> AFVVTDNCIKCKYTDCVEVCPVDCIYEGPNFLVIHPDECIDCALCEPECPAQAIFSEDEVPEDMQEFIQLNAELAEVWPN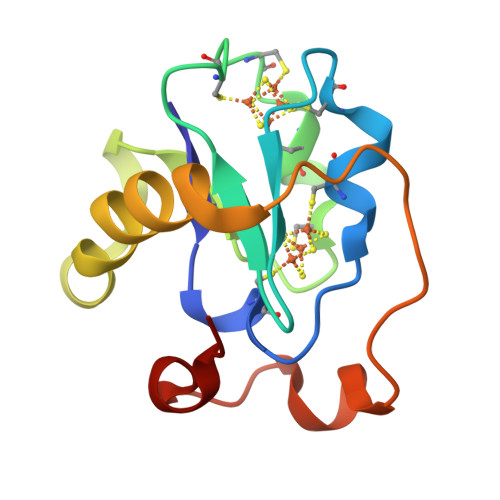ITEKKDPLPDAEDWDGVKGKLQHLER>MKDAHKVVWTEGMFLRPHHFQQAENYLEGYMRNWGQAHSGCFWGFLTLDLDQTLLRQGKIALNAASGIMPDGTPFRFSGAQQAPAPLAIADNKTGENVVLALPTYRAGREDVIFQESPEALARYLAYENEVDDLNAVSVGSAALQFGRLRLRLMLESELNAEWTALGVTRVLEKRGDNSLRLDTAQIPPMLNCQGNPVLKTFINDLQGLLQQRSQQMSQRLLQPGRGGSSEMVDFMLLQLINRHLGQVSHAYHLDHLHPERLFADWLQFATELASFSAQRTPEGRLPVYDHDNLALCFGKLMLL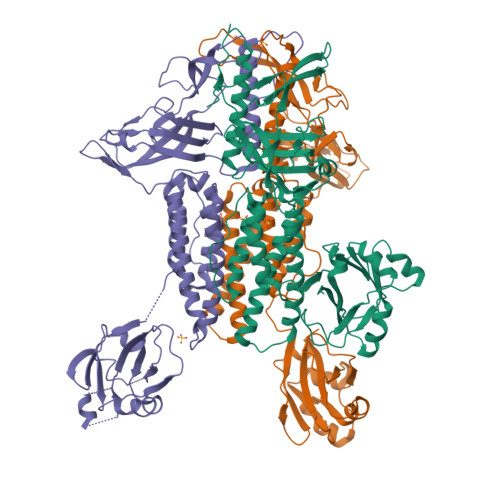LRQGLSVVLEDNAIQLTLVERSHGLNVATVQDTKMMRDFGFVLAVRADVAAEVLLTHFPAQMKIAPVTRIRDLVQLQLPGIGLRTMPVAPRQIPYHAGYTYFELEKGGDLWKQMEKSSAFALHLAGEFPGLDMEFWAIRSHTDRLEHHHHHH[3x]>SEDNIIGTTTQEIDEHGNVKTIITVKNQQIESYTSTDSGTAKNRSTLTVNANFLNDKYSNELTTILSLNGFIPSGRKFIFPKNNTLKGEMLWPQRYSTAVYNIPLDKSVKITNSTPDNTIRSKEVSNSITYGIGGGIKMEGKQPGANLDANAAITKTISYQQPDYETAKTTSTVTGVNWNTNFTETRDGYTRNSWNPVYGNQMFMYGRYTSNIRNNFTPDYQLSSLITSGFSPSYGLVLRAPKDVKKSRIKVVFARRSETYQQNWDGLNWWGRNFYDTKNPDSLSKVTLTFELDWQNHRVTFIELEH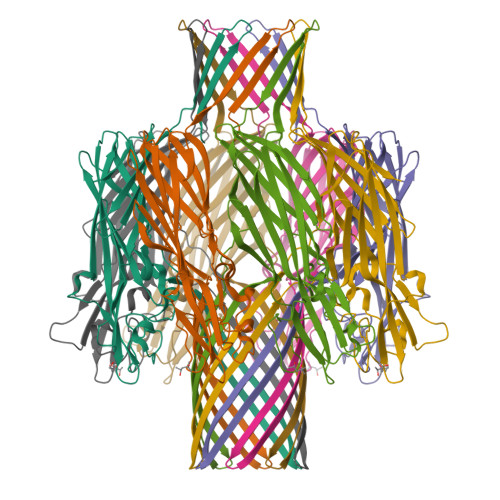HHHHH[2x]> CGVGFIAAIDGKPRRSVVEKGIEALKAVWHRGAVDADGKTGDGAGIHVAVPQKFFKDHVKVIGHRAPDNKLAVGQVFLPRISLDAQEACRCIVETEILAFGYYIYGWRQVPINVDIIGEKANATRPEIEQIIVGNNKGVSDEQFELDLYIIRRRIEKAVKGEQINDFYICSLSARSIIYKGMFLAEQLTTFYPDLLDERFESDFAIYHQRYSTNTFPTWPLAQPFRMLAHNGEINTVKGNVNWMKAHETRMEHPAFGTHMQDLKPVIGVGLSDSGSLDTVFEVMVRAGRTAPMVKMMLVPQALTSSQTTPDNHKALIQYCNSVMEPWDGPAALAMTDGRWVVGGMDRNGLRPMRYTITTDGLIIGGSETGMVKIDETQVIEKGRLGPGEMIAVDLQSGKLYRDRELKDHLATLKPWDKWVQNTTHLDE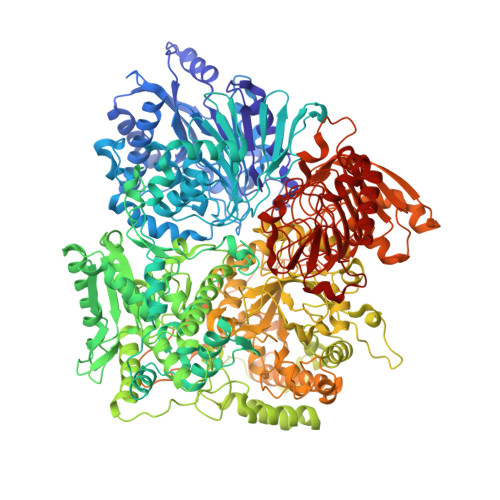LVKTASLKGEPSDMDKAELRRRQQAFGLTMEDMELILHPMVEDGKEAIGSMGDDSPIAVLSDKYRGLHHFFRQNFSQVTNPPIDSLRERRVMSLKTRLGNLGNILDEDETQTRLLQLESPVLTTAEFRAMRDYMGDTAAEIDATFPVDGGPEALRDALRRIRQETEDAVRGGATHVILTDEAMGPARAAIPAILATGAVHTHLIRSNLRTFTSLNVRTAEGLDTHYFAVLIGVGATTVNAYLAQEAIAERHRRGLFGSMPLEKGMANYKKAIDDGLLKIMSKMGISVISSYRGGGNFEAIGLSRALVAEHFPAMVSRISGIGLNGIQKKVLEQHATAYNEEVVALPVGGFYRFRKSGDRHGWEGGVIHTLQQAVTNDSYTTFKKYSEQVNKRPPMQLRDLLELRSTKAPVPVDEVESITAIRKRFITPGMSMGALSPEAHGTLNVAMNRIGAKSDSGEGGEDPARFRPDKNGDNWNSAIKQVASGRFGVTAEYLNQCRELEIKVAQGAKPGEGGQLPGFKVTEMIARLRHSTPGVMLISPPPHHDIYSIEDLAQLIYDLKQINPDAKVTVKLVSRSGIGTIAAGVAKANADIILISGNSGGTGASPQTSIKFAGLPWEMGLSEVHQVLTLNRLRHRVRLRTDGGLKTGRDIVIAAMLGAEEFGIGTASLIAMGCIMVRQCHSNTCPVGVCVQDDKLRQKFVGTPEKVVNLFTFLAEEVREILAGLGFRSLNEVIGRTDLLHQVSRGAEHLDDLDLNPRLAQVDPGENARYCTLQGRNEVPDTLDARIVADARPLFEEGEKMQLAYNARNTQRAIGTRLSSMVTRKFGMFGLQPGHITIRLRGTAGQSLGAFAVQGIKLEVMGDANDYVGKGLSGGTIVVRPTTSSPLETNKNTIIGNTVLYGATAGKLFAAGQAGERFAVRNSGATVVVEGCGSNGCEYMTGGTAVILGRVGDNFAAGMTGGMAYVYDLDDSLPLYINDESVIFQRIEVGHYESQLKHLIEEHVTETQSRFAAEILNDWAREVTKFWQVVPKEMLNRLEVPVHL> SEESRESPAEHGYYMPAEWDSHAQTWIGWPERQDNWRHNALPAQRVFAGVAKAISKFEPVTVCASPAQWENARKQLPEDIRVVEMSMNDSWFRDSGPTFIVRKRPVKLSSLNRNIAGIDWNFNAWGGANDGCYNDWSHDLLVSRKILALERIPRFQHSMILEGGSIHVDGEGTCLVTEECLLNKNRNPHMSKEQIEEELKKYLGVQSFIWLPRGLYGDEDTNGHIDNMCCFARPGVVLLSWTDDETDPQYERSVEALSVLSNSIDARGRKIQVIKLYIPEPLYMTEEESSGITQD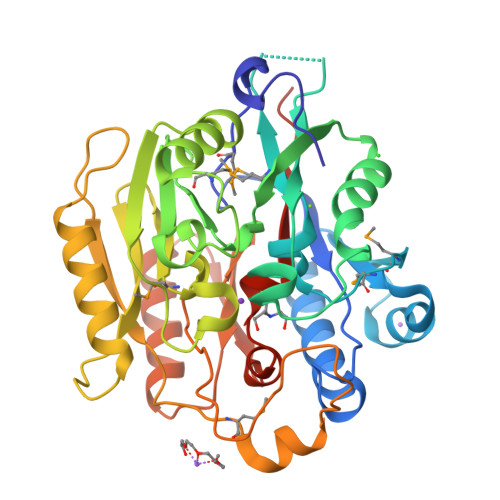GEAIPRLAGTRLAASYVNFYIANGGIIAPQFGDPIRDKEAIRVLSDTFPHHSVVGIENAREIVLAGGNIHCITQQQPAEPTSVAENGH> NTYQFRNMIECTVPSR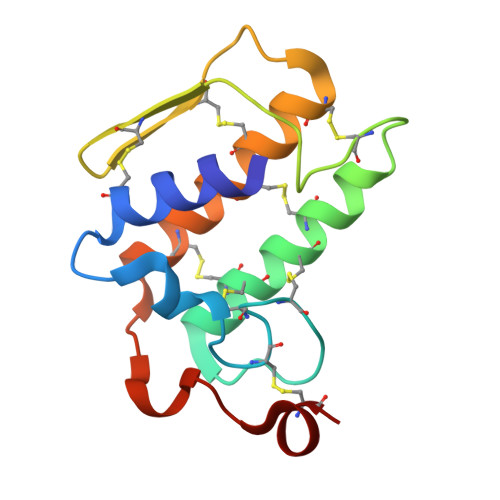SWWDFADYGCYCGCGSGTPTDDLDRCCQVHCNCYRQAGEISGCRPKFKTYTYQCSGGTLTCKGNNNACAASSCDCDRLAAICFAGAPYNDNNYNIDLKARCN>[4x]VLDGPYQPTNFKPPNDYWILLNPTNQQVVLEGTNKTDIWVA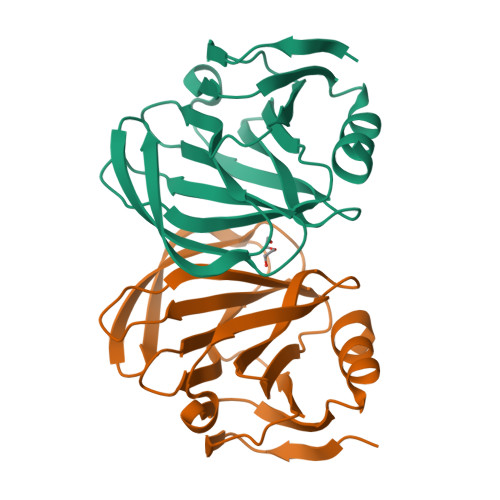LLLVEPNVTNQSRQYTLFGETKQITVENNTNKWKFFEMFRSNVSAEFQHKRTLTSDTKLAGFMKFYNSVWTFHGETPHATTDYSSTSNLSEVETVIHVEFYIIPRSQESKCSEYINTG>MASTDYHVDLTNCDREPIHIPGYIQPHGCLIACDNAMRMVLRHSENCGELLGLEGDLNGRTAEDVLGKRLVHDLRNALTVTGKTTRPAMLPAMETSDGRSFDISLHRYKSTTIIEFEPSDSDTQPLGTARKMVDRIREADSVESLISRTTRLVKATLGYDRVLIYRFEEDGAGKVVSEAKQPELESFLGQYFPASDIPQQARALYLKNTLRIISDASGTPIPVLPAVDVSGEPLDLSYAHLRNFSPIHCEYLRNMGVAASMSISVIVDDALWGLIVCHHCSPRVLSMPVRIAAAMFGEFFSMFLQVLKQKRRLDTINHAHAALDRFLRLAAHRANLEELLVDSFQDFARLIPCDGVGLWVGNNWHGHGATPPHDAIPRLARFVASVSEGRVWATHALSQAIPEAEIYADTAAGMLAIPISQVKSDYLLFFRKEIVQNLNWAGNPEKSYETGPMGDRLTPRKSFAIWKESVRLQAQPWSEADREIAETARIALVGVAFHHSELMAGLEYK[2x]

Phytochromes are biliproteins of plants, bacteria and fungi that use red light as a source of information to regulate fundamental physiological processes, such as photosynthesis, seed germination, flowering and shade avoidance. The molecular architecture of phytochromes shares a common photosensory core module (PCM), which is composed of PAS (Per/Arnt/Sim), GAF (cGMP phosphodiesterase/adenyl cyclase/FhlA) and PHY (phytochrome-specific) domain4–6. Bacterial phytochromes can be grouped into prototypical and bathy phytochromes, in which the red-absorbing Pr and far-red-absorbing Pfr are the thermodynamically stable states, respectively. The conjugate Meta-F and Pfr crystal structures has been obtained from the engineered photoactivatable near-IR fluorescent protein (Agp2-PAiRFP2), derived from the bathy phytochrome Agp2 from Agrobacterium fabrum.

Preliminary crystallization and spectroscopic experiments identified the PCM fragment of the photoactivatable phytochrome Agp2-PAiRFP2 as a promising candidate. The half-lives of the photoinduced states of Agp2-FL, Agp2-PCM and the PCM fragment of Agp2-PAiRFP2 are 170 s11, 20 s11 and 233 min, respectively. This Agp2-PCM variant includes 24 substitutions, which except for Val244Phe and Ala276Val do not participate in the interaction between the chromophore and chromophore-binding site. Agp2-PAiRFP2 was crystallized in the dark adapted Pfr state (in the hexagonal space group P6322) and the structure was solved at a resolution of 2.03 Å. Remarkably, crystal packing and crystallization conditions differ significantly from those of Agp2-PCM. While Agp2-PCM shows a parallel orientation of the two crystallographic monomers, Agp2-PAiRFP2 monomers crystallize in a near anti-parallel arrangement. However, the overall topologies of the monomers in both structures agree very well, as demonstrated also by superposition of the equivalent Cα atoms of both constructs yielding a root-mean-square deviation of only 0.6 Å. Also, structural details of the chromophore pocket are very similar, including the ZZEssa stereochemistry of BV and the exocyclic double bond of ring A of the chromophore, which results in sp3 hybridization of the C2 atom and therefore an out-of-plane oriented bond to the methyl group at this position. The chromophore interaction interface to the surrounding amino acids, especially potential hydrogen bonds, hydrophobic interactions and water molecules, are almost identical for the Pfr states of both Agp2-PCM variants. Ultraviolet–visible absorption spectra of Agp2-PAiRFP2 compared to the wild-type Agp2-PCM construct, the full-length Agp2 (Agp2-FL) and the prototypical full-length phytochrome Agp1 (Agp1-FL) display the characteristic spectrum of Pfr but an enhanced stability of the final photoproduct state, resulting in slower dark reversion to Pfr compared to Agp2-PCM.>[2x]EGHAGGIGIAEFLGGKNFLITGGTGFLAKVLIEKILRTNPDVGKIYVLIKAKDGDAALKRLHNEVVDTELFSRLQEIHGKDYHSFAARKLVPVVGDVREANVGIAPELAGVIADEVDIIVNSAANTTFDERYDVAMDINTVGPFRIMSFAQRFRRLKLFLQVSTAYVNGQRQGVVLEKPFRLGDTIAKELGSPDSSQHKNTMLDIEAEIKLAFDHRRHGDDSASFSEEMKELGLERAKLHGWQDTYVFTKAMGEMVINSM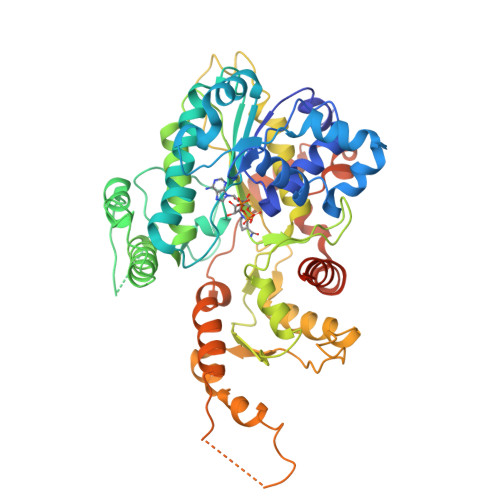RGDIPVVTIRPSVIESTWRDPFPGWMEGNRMMDPVVLYYGKGQLSGFLADPEGVLDVVPADMVVNATLASMAKHGRGGAAAAAAAAEGMHVYHVASSTVNPLAFGDLSRFLFQHFTGSPYSDAAGRPIHVPPMRLFDTMEQFASYVETDALLRAGRLAGAGAGAGDERVSQRLRELCAKSVEQTIYLGSIYQPYTFYGGRFDNGNTEALIGEMSEEEKARFHFDVRSIEWTDYITNVHIPGLRKHVMKGRGVGGGSGASSSSNASLLAGASV>[3x]HQSQLDRERILSLEQRVVELQQTLAQKDQALGKLEQSLRLMEEASFDGTFLWKITNVTRRCHESACGRTVSLFSPAFYTAKYG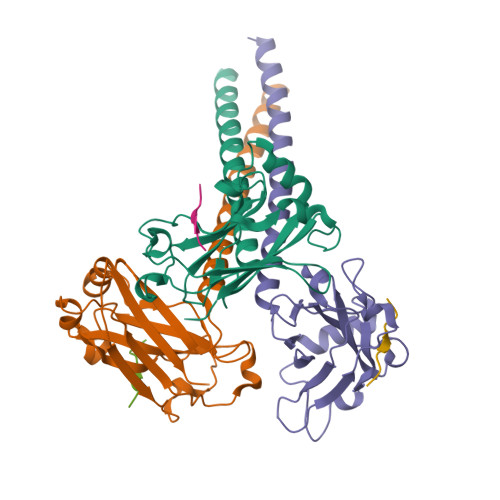YKLCLRLYLNGDGTGKRTHLSLFIVIMRGEYDALLPWPFRNKVTFMLLDQNNREHAIDAFRPDLSSASFQRPQSETNVASGCPLFFPLSKLQSPKHAYVKDDTMFLKCIVETSTLEHHHHHH;>[3x]SVPIQCTD> IVGGYICEENSVPYQVSLNSGYHFCGGSLISEQWVVSAGHCYKSRIQ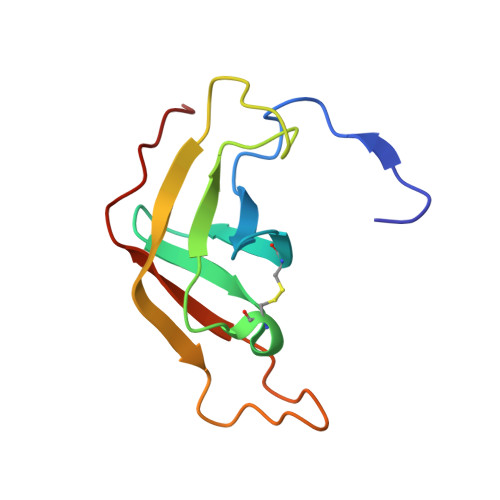VRLGEHNIEVLEGNEQFINAAKIIRHPKYNSRTLDNDILLIKLSSPAVINSR> GAMDPGNSAEAWKNLGNAYYKQGDYQKAIEYYQKALELDPNNASAWYNLGNAYYKQGDYQKAIEYYQKALELDPNNAKAWYRRGNAY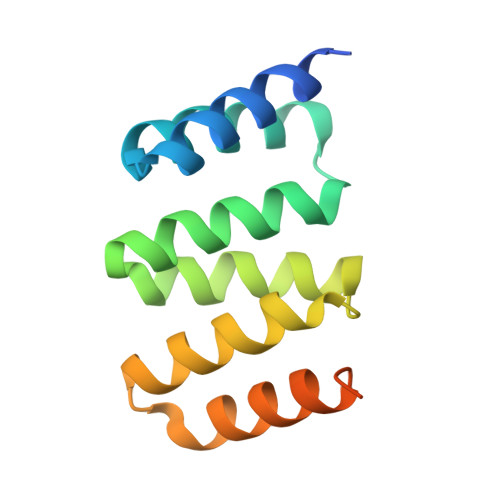YKQGDYQKAIEDYQKALELDPNNAKAKQNLGNAKQKQG>MIYFRSVFLATCLLCSGIGASVYAAMPSSQDNGSAEVIELFFSAAKVGNIEVLQEFLSHGFPIDVQDHSGYTALMMASYYGQKDAVKVLLEQGANRCLRDKRGHTALMGAIVKAEWGIAKQLRQV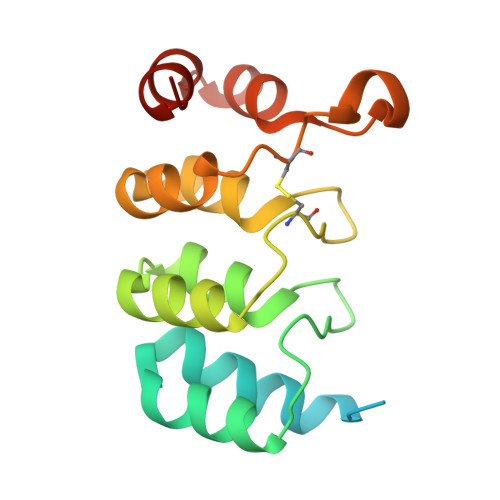DCDANAAKTGLLTAEQFAIQFGQQQRLKDIQPSTEK[4x]2,4-dimethoxypyrimidine | C6 H8 N2 O2 | 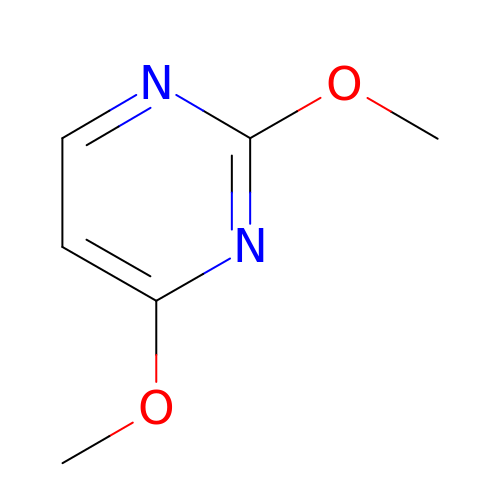KEVRHVMWBKFGLO-UHFFFAOYSA-N>[4x]MSLTKIDAYAHILPAKYYQKMLSVEPNIPNMFPFIKIKTLMDLDERLTKWPDQNTKQVISLANISPEDFTDSKTSAELCQSANEELSNLVDQHPGKFAGAVAIL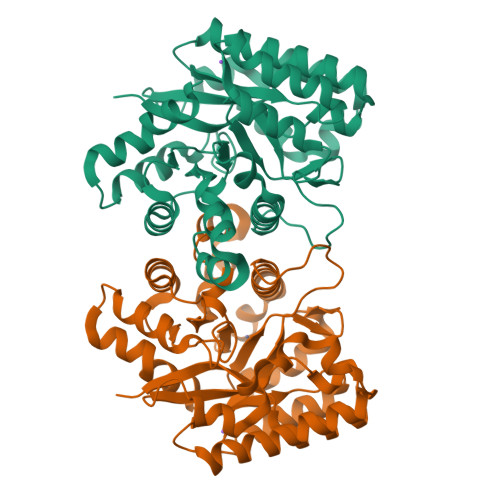PMNNIESACKVISSIKDDENLVGAQIFTRHLGKSIADKEFRPVLAQAAKLHVPLWMHPVFDARKPDNNLVFSWEYELSQAMLQLVQSDLFQDYPNLKILVHHAGAMVPFFSGRIDHILDEKHAQDFKKFYVDTAILGNTPALQLAIDYYGIDHVLFGTDAPFAVMPSGADQIITQAINDLTISDKDKQKIFHDNYYSLIKEGHHHHHH> QECTKFKVSSCRECIESGPGCTWCQKLNFTGPGDPDSIRCDTRPQLLMRGCAADDIMDPTSLAETQEDHNGGQKQLSPQKVTLYLRPGQAAAFNVTFRRAKLSSRVFLDHNALPDTLKVTYDSFCSNGVTHRNQPRGDCDGVQINVPITFQV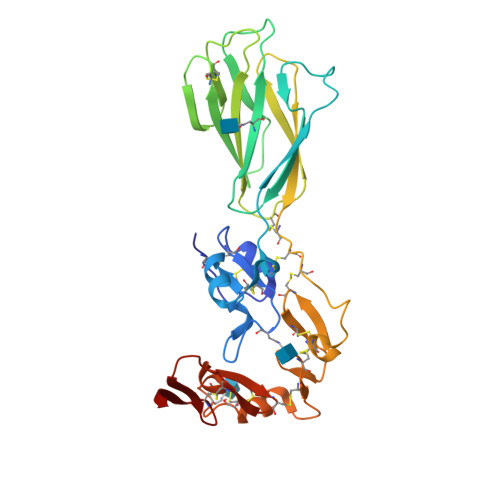KVTATECIQEQSFVIRALGFTDIVTVQVLPQCECRCRDQSRDRSLCHGKGFLECGICRCDTGYIGKNCECQTQGRSSQELEGSCRKDNNSIICSGLGDCVCGQCLCHTSDVPGKLIYGQYCEHHHHHH>GELLDPCGYISPESPVVQLHSNFTAVCVLKEKCMDYFHVNANYIVWKTNHFTIPKEQYTIINRTASSVTFTDIASLNIQLTCNILTFGQLEQNVYGITIISGLPPEKPKNLSCIVNEGKKMRCEWDGGRETHLETNFTLKSEWATHKFADCKAKRDTPTSCTVDYSTVYFVNIEVWVEAENALGKVTSDHINFDPVYKVKPNPPHNLSVINSEELSSILKLTWTNPSIKSVIILKYNIQYRTKDASTWSQIPPEDTASTRSSFTVQDLKPFTEYVFRIRCMKEDGKGYWSDWSEEASGITYED[6x];>[6x]GPGPPPGPPRVSPDPRAELDSTVLLTRSLLADTRQLAAQLRDKFPADGDHNLDSLPTLAMSAGALGALQLPGVLTRLRADLLSYLRHVQWLRRAGGSSLKTLEPELGTLQARLDRLLRRLQLLMSRLALPQPPPDPPAPPLAPPSSAWGGIRAAHAILGGLHLTLDWAVRGLLLLKTRL;>[6x]SSPCPQAWGPPGVQYGQPGRSVKLCCPGVTAGDPVSWFRDGEPKLLQGPDSGLGHELVLAQADSTDEGTYICQTLDGALGGTVTLQLGYPPARPVVSCQAADYENFSCTWSPSQISGLPTRYLTSYRKKTVLGADSQRRSPSTGPWPCPQDPLGAARCVVHGAEFWSQYRINVTEVNPLGASTRLLDVSLQSILRPDPPQGLRVESVPGYPRRLRASWTYPASWPSQPHFLLKFRLQYRPAQHPAWSTVEPAGLEEVITDAVAGLPHAVRVSARDFLDAGTWSTWSPEAWGTPSTGTIPKEIPAWGQLHTQPEVEPQVDSPAPPRPSLQPHPRLLDHRDSVHHHHHHH

Interleukin (IL-), an IL-6 family cytokine, has pivotal roles in autoimmune diseases, fibrotic complications, and solid cancers. IL-11 activates downstream signalling pathways by binding its two cell surface receptors: the IL-11 specific receptor, IL-11Rα, and the signal-transducing receptor, glycoprotein (gp)13013,26. Following the formation of the receptor complex, the Janus kinase (JAK)/signal transducer and activator of stat (STAT) and extracellular signal regulated kinase (ERK)/mitogen-activated protein kinase (MAPK) pathways are primarily activated. IL-11 and IL-6 utilise a homodimer of gp13026,34,35 while other IL-6 family members exploit a heterodimer of gp130 with a second signal-transducing receptor, such as LIF receptor (LIFR), OSM receptor (OSMR), IL-27R/WSX-1 or IL-12 receptor β−2 subunit (IL-12Rβ2).

To understand the molecular mechanisms underpinning human IL-11 signalling complex formation, we solved three structures of the complex containing either the cytokine binding domains of gp130 (gp130D1-D3) or the complete extracellular domains of gp130 (gp130EC) using electron cryo-microscopy (cryo-EM) and X-ray crystallography. We also obtained crystals of the IL-11FL/IL-11RαEC/gp130D1-D3 complex that diffracted anisotropically to 3.8 Å. We used the cryo-EM structure of the gp130D1-D3 complex to phase the X-ray diffraction data by molecular replacement. Three IL-11 signalling complexes were arranged in a triangular configuration in the asymmetric unit providing 6-fold non-crystallographic symmetry to aid refinement. Satisfactory density defining the positions of the β-sheets of IL-11Rα D1 facilitated refinement of the domain in the gp130EC complex and the crystal structure, confirming the average positions of this domain in the complex. N-linked glycans were visible on IL-11Rα (N105, N172) and gp130 (N21, N61, N135) in all structures.> MGWSLPKEKGLILCLWNKFCRWFHRRESWAQSRDEQNLLQQKRIWESPLLLAAKENNVQALYKLLKFEGCEVHQKGAMGETALHIAALYDNNEAAQVLMEAAPELVFEPMTSELYEGQTALHIAVINQNVNLVRALLARGASVSARATGSVFHYRPHNLIYYGEHPLSFAACVGSEEIVRLLIEHGADIRAQDSLGNTVLHILILQPNKTFACQMYNLLLSYDGGDHLKSLELVPNNQGLTPFKLAGVEGNIVMFQHLMQKRKHIQWTYGPLTSTLYDLTEIDSSGDDQSLLELIVTTKKREARQILDQTPVKELVSLKWKRYGRPYFCVLGAIYVLYIICFTMCCVYRPLKPRITNRTNPRDNTLLQQKLLQEAYVTPKDDLRLVGELVSIVGAVIILLVEIPDIFRLGVTRFFGQTILGGPFHVIIVTYAFMVLVTMVMRLTNSDGEVVPMSFALVLGWCNVMYFARGFQMLGPFTIMIQKMIFGDLMRFCWQMAVVILGFASAFYIIFQTEDPDELGHFYDYPMALFSTFELFLTIIDGPANYDVDLPFMYSITYAAFAIIATLLMLNLLIAMMGDTHWRVAHERDELWRAQVVATTVMLERKLPRCLWPRSGICGREYGLGDRWFLRVEDRQDLNRQRIRRYAQAFQQQDDLYSEDLEKDSGEK

TRPV6 and its close relative TRPV5 are TRP channels that are distinctly Ca2+-selective and play an important role in calcium homeostasis. Structurally, TRP channels are assemblies of four identical subunits arranged symmetrically around the pore axis. The transmembrane domain of TRP channels includes six transmembrane helices (S1–S6) and a pore loop (P-loop) between S5 and S6. S5, P-loop and S6 form the KcsA channel-like pore domain, with the ion conduction pathway lined by the S6 helices and extracellular loops connecting the P-loop helix to S5 and S6.

Compared to wild type, TRPV6cryst has a 59-residue C-terminal truncation and four point mutations, including L495Q, which resides in the S5 transmembrane helix. This L495Q substitution, which was a spontaneous mutation that occurred during gene synthesis, was originally included in TRPV6cryst because it expressed at 3-fold higher levels than the same construct with the substitution reverted to the native leucine (TRPV6*). We reproduced crystals of TRPV6cryst and confirmed its non-swapped conformation. Notably, we were able to collect new crystallographic data, where both the S4–S5 and S6-TRP helix connectivity in TRPV6cryst is unambiguously resolved in the 2Fo-Fc and Fo-Fc omit maps, in stark contrast to our previous data, where density for thirteen residues in S4–S5 linker (F471-Q483) was missing. Similarly, both the 2Fo-Fc and robust Fo-Fc omit maps for TRPV6* demonstrated completely different connectivity of transmembrane domains compared to TRPV6cryst. These structural data therefore suggest that the single leucine L495 to glutamine substitution in S5 is responsible for the absence of domain swapping in TRPV6cryst. By contrast, in TRPV6cryst, Q495 is rotated by ~120° with respect to the orientation of L495 in TRPV6* and forms polar interactions with the hydrophilic pocket formed by S4–S6 and the TRP helix of the same subunit. Disruption of these hydrophobic interactions leads to the non-swapped fold. Apart from the distinct connectivity between S4 and S5 as well as S6 and TRP helix, the domain-swapped TRPV6* and non-swapped TRPV6cryst structures were almost identical. Despite these gross similarities, kinetic analysis indicated the rate of increase in Fura-2 signal is faster in TRPV6* compared to TRPV6cryst. Therefore, the Ca2+ entry function is somewhat compromised in the non-swapped TRPV6cryst construct, presumably due to differences in allosteric communication between the pore domain and the rest of the protein.>[2x]KSVAHHEDVYSHNLPPMDEKEMALYKLYRPERVTPKKRSAELLKEPRLNKGMGFSLYERQYLGLHGLLPPAFMTQEQQAYRVITKLREQPNDLARYIQLDGLQDRNEKLFYRVVCDHVKELMPIVYTPTVGLACQNFGYIYRKPKGLYITINDNSVSKIYQILSNWHEEDVRAIVVTDGERILGLGDLGAYGIGIPVGKLALYVALGGVQPKWCLPVLLDVGTNNMDLLNDPFYIGLRHKRVRGKDYDTLLDNFMKACTKKYGQKTLIQFEDFANPNAFRLLDKYQDKYTMFNDDIQGTASVIVAGLLTCTRVTKKLVSQEKYLFFGAGAASTGIAEMIVHQMQNEGISKEEACNRIYLMDIDGLVTKNRKEMNPRHVQFAKDMPETTSILEVIRAARPGALIGASTVRGAFNEEVIRA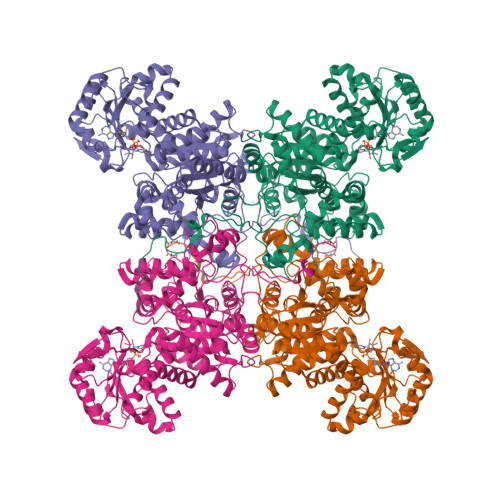MAEINERPIIFALSNPTSKAECTAEEAYTFTNGAALYASGSPFPNFELNGHTYKPGQGNNAYIFPGVALGTILFQIRHVDNDLFLLAAKKVASCVTEDSLKVGRVYPQLKEIREISIQIAVEMAKYCYKNGTANLYPQPEDLEKYVRAQVYNTEYEELINATYDWPEQDMRHGFPVPVVRHDSMDG> 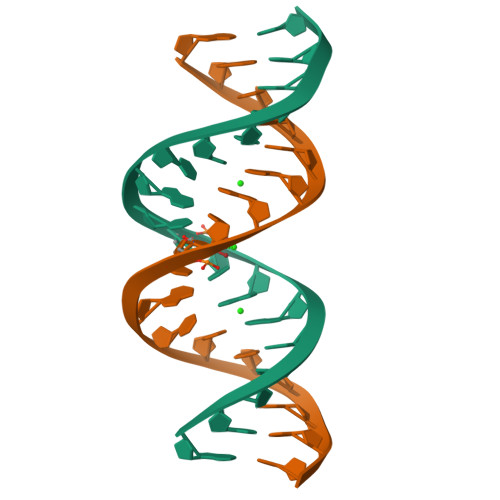GGTGGGGCUTGCCCCACC> MLNSFKLSLQYILPKLWLTRLAGWGASKRAGWLTKLVIDLFVKYYKVDMK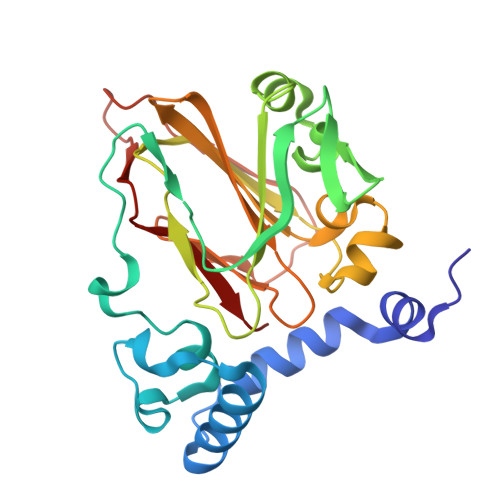EAQKPDTASYRTFNEFFVRPLRDEVRPIDTDPNVLVMPADGVISQLGKIEEDKILQAKGHNYSLEALLAGNYLMADLFRNGTFVTTYLSPRDYHRVHMPCNGILREMIYVPGDLFSVNHLTAQNVPNLFARNERVICLFDTEFGPMAQILVGATIVGSIETVWAGTITPPREGIIKRWTWPAGENDGSVALLKGQEMGRFKLG> MAPITAYSQQTRGL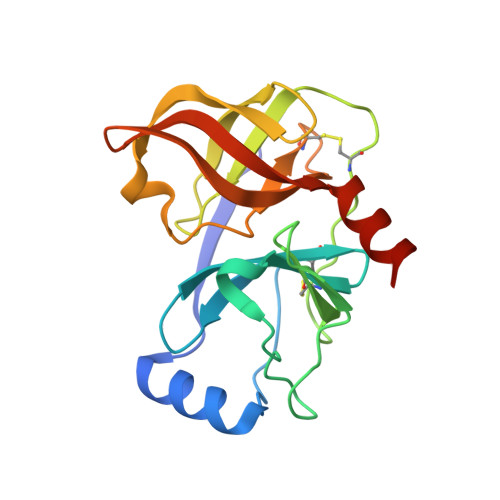LGCIITSLTGRDKNQVDGEVQVLSTATQSFLATCVNGVCWTVYHGAGSKTLAGPKGPITQMYTNVDQDLVGWPAPPGARSMTPCTCGSSDLYLVTRHADVIPVRRRGDSRGSLLSPRPVSYLKGSSGGPLLCPSGHVVGIFKAAVCTRGVAKAVDFIPVESMETTMRASKKKK> PHMENEDFCAVCLNGGELLCCDRCPKVFHLSCHVPALTSFPGGEWVCTLCRSLTQPEMEYDSENASHNQPGKRASPGLSMYDQKKCEKLVLSLCCNNLSLPFHEPVSPLARHYYQIIKRPMDLSTIRRKLQKKDPAHYTTPEEVVSDVRLMFWNCAKFNYPDSEVAEAGRSLENFFEGWLKEIYPEKRFAQPRQED

The paralog of TRIM24, TRIM28, and TRIM33—termed TRIM66—also contains a PHD-Bromodomain at its C terminus. Herein, we determine the crystal structure of the TRIM66 PHD-Bromodomain in its free state and in a complex with the N terminus of histone H3. Our results show that the PHD domain of TRIM66 recognizes both unmodified H3R2 and H3K4 residues, whereas the Bromodomain interacts with the H3K56ac peptide through its ZA and BC loops. Further studies show that TRIM66 regulates the deacetylation of H3K56ac by recruiting histone deacetylase Sirt6, providing the appropriate chromatin environment for subsequent DNA repair and safeguarding the genomic integrity of ESCs.

We used the mutant TRIM66-MUT968-1160 protein for the crystallization experiment and determined the crystal structure of the TRIM66 PHD-Bromodomain in free state. The 2.1 Å crystal structure of the TRIM66 PHD-Bromodomain showed that the PHD domain adopted a typical cross-braced topology, whereas the Bromodomain adopted a typical left-handed four-helical bundle topology. There was an extensive interface between the PHD and Bromodomain, enabling the formation of a unified structural unit. The results showed that the H3K56ac peptide interacted with the ZA and BC loops of the TRIM66 Bromodomain. Residues F1122, N1123, Y1124, and D1126, which exhibited the most obvious perturbations, were all located on the BC loop, whereas V1070, S1071, Y1078, Q1079, I1080, and I1081 were located on the ZA loop. One asparagine on the BC loop (N1123 in TRIM66) was conserved and played critical roles in recognizing acetyl-lysine.> MGSSHHHHHHSSGRENLYFQGMVESKNTELSQGTWLNKPKSVFQEAGKVTLETDEKTDFWRETFYGFTRDSGHFLGV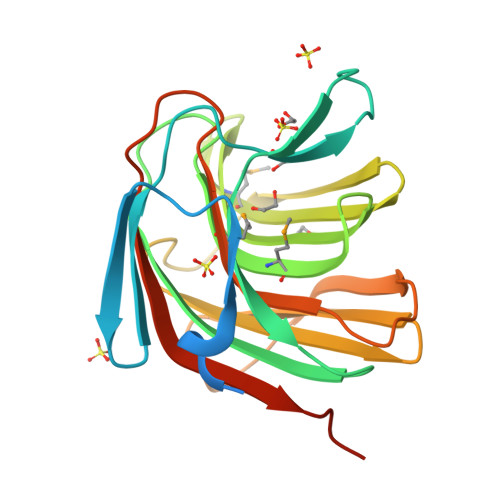ETGSAFTAQVRVQGSYESLYDQAGIMVRIDDGHWLKAGIEISDGHAMLSSVLTNGKSDWSTAVYGGNARDFWLRVTVEKGVLRIQVSSDKKTWPLVRLAPFPTSDHYLVGPMACTPERGGLKVTFSEWSLTAPLGKALHDLSGS>MNYARFITAASAARNPSPIRTMTDILSRGPKSMISLAGGLPNPNMFPFKTAVITVENGKTIQFGEEMMKRALQYSPSAGIPELLSWLKQLQIKLHNPPTIHYPPSQGQMDLCVTSGSQQGLCKVFEMIINPGDNVLLDEPAYSGTLQSLHPLGCNIINVASDESGIVPDSLRDILSRWKPEDAKNPQKNTPKFLYTVPNGNNPTGNSLTSERKKEIYELARKYDFLIIEDDPYYFLQFNSGRVPTFLSMDVDGRVIRADSFSKIISSGLRIGFLTGPKPLIERVILHIQVSTLHPST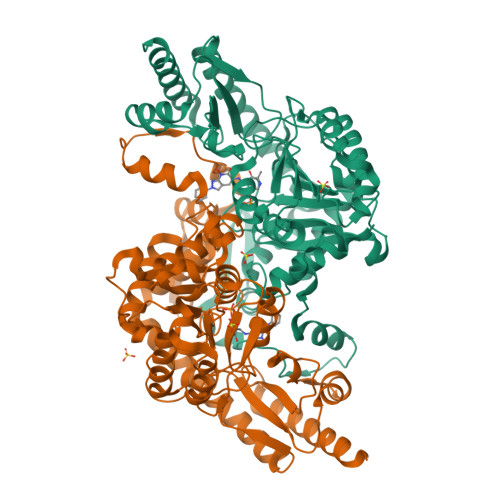FNQLMISQLLHEWGEEGFMAHVDRVIDFYSNQKDAILAAADKWLTGLAEWHVPAAGMFLWIKVKGINDVKELIEEKAVKMGVLMLPGNAFYVDSSAPSPYLRASFSSASPEQMDVAFQVLAQLIKESLLVPRGSLEHHHHHH[2x]The β-barrel assembly machinery (BAM) complex is a conserved, multiprotein machine that mediates the folding and membrane insertion of newly synthesized β-barrel outer membrane (OM) proteins. Cryogenic electron microscopy (cryo-EM) structures of the BAM complexes from the gut commensal B. thetaiotaomicron and the oral pathogen Porphyromonas gingivalis are similar and reveal a 7-protein, ~325-kDa complex with most of its mass on the extracellular side. Remarkably, besides BamA and BamD subunits, Bacteroidetal BAM contains a 14-stranded integral OMP that is intimately associated with BamA. The remaining four components, named BamH–K, are all SLPs and form an extracellular dome-like structure over BamA that may provide additional functionality to enable the folding and assembly of the many β-barrel–SLP complexes that are a hallmark of the Bacteroidota.

Class 1 lacks density for the periplasmic components but has good density for all extracellular proteins, whereas class 2 has modest resolution for BamA POTRA domains 4 and 5 and for part of BamD, but with poorly resolved extracellular areas. The 14-stranded barrel of the integral membrane component BamG occupies a key position within BtBAM. It forms a tight complex with the back of BamA (defined as being located opposite the BamA lateral gate), with an interface area of ~1,560 Å2 as analysed via PISA33, and binds Bt4306 (renamed BamH) via its extracellular loops (interface area ~1,720 Å2). A feature that clearly distinguishes BamG from FadL channels with a known transport role is an extension of the N-terminus of ~10 residues, which protrudes through the lateral opening in the barrel wall that normally is part of the FadL transport pathway. Similarly to Proteobacterial BAM complex structures, the cryo-EM maps suggest considerable heterogeneity and/or mobility within BamA and BamD. Density for BamA POTRA domains 1–3 and for the N-terminal region of BamD is missing (residues 18–71), and the visible periplasmic components have a relatively low resolution. Likewise, density for β1 and β2 strands of BamA is poor, suggesting heterogeneity at the lateral gate and a loose association of β1 and β16 strands. BtBamA has a striking extracellular loop (EL) 3 between the β5 and β6 strands, which contains 13 tyrosine residues and probably projects inside the dome formed by the SLPs. There was no cryo-EM density observed for this 38-residue loop, which suggests that it samples a range of different conformations.

> MHYRISFIFVTFICLFCFAATGFTQNTNHHHHHHHTDEDSKPVILYSGTPKKYEIADIKVEGVKNYEDYVLIGLSGLSVGQTITVPGDEITGAIKRYWKHGLFSNVQITAEKIEGNKIWLKISLTQRPRIADVRYHGVKKSERTDFESKLGMVKGMQITPNTVDRAKTLIKRYFDDKGFKNAEVIIAQKDDPSNENQVIVDIDIDKKEKIKVHAIHITGNSAIKTSKLKKVMKKTNEKGKLLNLFRTKKFVPENFEADKQLIIDKYNELGYRDAMIVKDSVAQYDEKTVDVYMDIDEGQKYYLRNVTWVGNTLYPSEQLNFLLRMKKGDVYNQKLLGERTSTDDDAIGNLYYNNGYLFYNLDPVEVNIVGDSIDLEMRIYEGRQATINKINISGNDRLYENVVRRELRIRPGQLFSKDDLMRSLREIQQMGHFDPEKLQPDIQPDPVNGTVDIGLPLTSKANDQVEFSAGWGQTGIIGKLSLKFTNFSVANLLRPGENYRGILPQGDGQTLTISGQTNAKYYQSYSISFFDPWFGGKRPNSLSVSAFFSVQTDISSRYYNSSYFNNYYNSMYSGYGGYGMYNYGNYNNYENYYDPDKSIKMWGLSLGWGKRLKWPDDYFTLSAELAYQRYNLKDWQYFPVTNGKCNDLSLSLTLARNSIDNPIFPRTGSDFSLSVQLTPPYSLFDGKDYKGYFYDPTDDRGITQDNMNKLHRWVEYHKWKFKAKTYTPLMDYIAHPKCLVLMTRTEFGLLGHYNKYKKSPFGTFDVGGDGMTGYSSYATESIALRGYENSSLTPYGKEGYAYARLGIELRYPLMLETSTNIYVLGFLEAGNAWHDISKFNPFDLKRSAGIGVRIFLPMIGMMGIDWGYGFDKINGSKEYGGSQFHFILGQEF;> MKKNIIITLLAAASLTSCGEYNKLLKSTDYEYKYEAAKNYFAKGQYNRSATLLNELITILKGTDKAEESLYMLGMSYYNQKDYQTAAQTFITYFNTYPRGTFTELARFHAGKSLFLDTPEPRLDQSSTYQAIQQLQMFMEYFPNSTKKQEAQDMIFALQDKLVLKELYSAKLYYNLGNYLGNNYESCVITAQNALKDYPYTDYREELSILILRARHEMAIYSVEDKKMDRYRETIDEYYAFKNEFPESKYLKEAEKIFNESQKVIKD;> MVGFKHTIWALLLMMVTGTAIAQNNTNSPYTRYGYGDLSDQSFGNSKAMGGIAFGLRDGAQINPTNPASYTAIDSLTFLFEGGVSLQNMNISGGGLKLNAKNASFDYLAMQFRLAPWMAMSVGLLPYSNVGYTVSDSQTTDNGLAYSRSFTGDGGLHQMYVGAGVKVLKNLSVGVNASYFWGDITRTRGMFYPGTSSYDSYQRKMVTSISDYKLDFGAQYTQALNKKSSLTIGAVYSPKHKLNNDYTSIVIMGASSSSYGTEYKDVLDATFELPNTFGVGFTYNYDKRLTVGADYSLQQWSKTNFGVVTSDENVRQDFNETFTYCDRTKISVGAEYIPNLIGRSYFAHIKYRLGAYYTTPYYKIDGKKASREYGVTAGFGLPVPRSRSILSISGQFVRVKGLETNMVNENIFRVSIGLTFNERWFFKRRVE O-benzyl-N-(benzylsulfonyl)-D-seryl-N-[(4-carbamimidoylphenyl)methyl]glycinamide 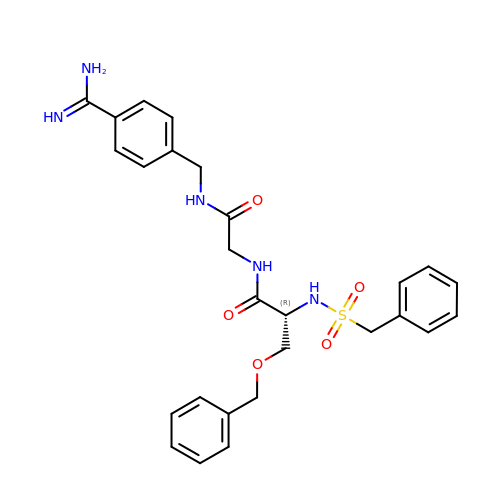| C27 H31 N5 O5 S | RXJPCNAPBKYKMA-XMMPIXPASA-N> MMDRCLIVFDLDTKLLEQHYHNSSWRNGYADIQRVLYRHRFNNIQGTVYLSERGVRQAHGTLALQEVAIRFQWFDKCVSNVQFYDLSDDFNAQFIIDGVTQAREAFERRIGMLRHQLLDAGLTSEKIEEIIGQQKFSLENATQIALPNPD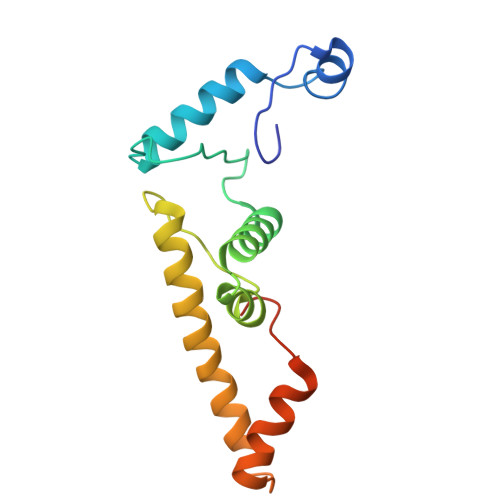D> MSLESVKAMWGVVTDSQTEIVALAKVRNEDVVPIVVSGYHYTIEMNGVKVADGYENSPVTVKPASATTLKFSLRLNNSFLREWWVTHIANGEKTKIRVAIKPTIEIGGRDVEVPVFLR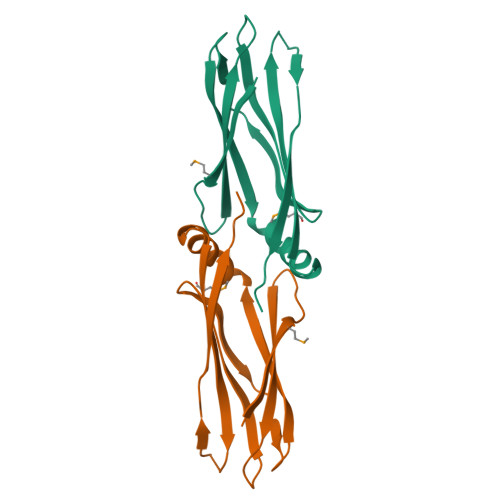ESEFTTKLLSEGHHHHHH>DNDDYDEKPREECGVVGIYGDSEASRLCYLALHALQHRGQEGAGIVTVSKDKVLQTITGVGLVSEVFSESKLDQLPGDIAIGHVRYSTAGSSMLKNVQPFVAGYRFGSVGVAHNGNLVNYTKLRADLEENGSIFNTSSDTEVVLHLIAISKARPFFMRIVDACEKLQGAYSMVFVTEDKLVAVRDPHGFRPLVMGRRSNGAVVFASETCALDLIEATYEREVYPGEVLVVDKDGVKCQCLMPHPEPKQCIFEHIYFSLPNSIVFGRSVYESRHVFGEILATES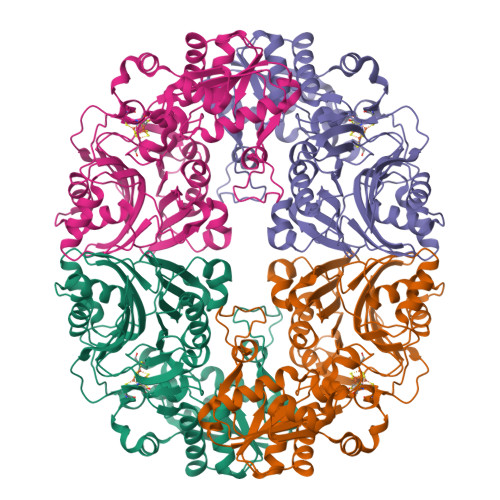PVDCDVVIAVPDSGVVAALGYAAKAGVAFQQGLIRSHYVGRTFIEPSQKIRDFGVKLKLSPVRGVLEGKRVVVVDDSIVRGTTSSKIVRLLREAGAKEVHMRIASPPIIASCYYGVDTPSSNELISNRMSVDEIRDYIGCDSLAFLSFETLKKHLGEDSRSFCYACFTGDYPVKPTEDKVKRGGDFIDDGLVGGIHNIEGGWVR[2x]> ENNPEEELASKQKNEESKKRQWALEDFEIGRPLGKGKFGNVYLAREKQSKFILALKVLFKAQLEKAGVEHQLRREVEIQSHLRHPNILRLYGYFHDATRVYLILEYAPLGTVYRELQKLSKFDEQRTATYITELANALSYCHSKRVIHRDIKPENLLLGSAG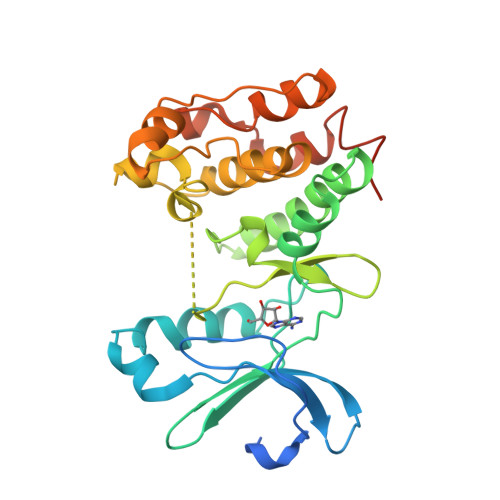ELKIADFGWSVHAPSSRRTTLCGTLDYLPPEMIEGRMHDEKVDLWSLGVLCYEFLVGKPPFEANTYQETYKRISRVEFTFPDFVTEGARDLISRLLKHNPSQRPMLREVLEHPWITANSSKPSNCQNKESASKQS>GHMSHWIWQHKDWPHFFWDEKLLSSHLSSARLVQGKLLGIIHTINQQTARQMNAFVLADQAVDTSAIEGEHLNRDSVRSSIANRLGLKQVGINKPVDRYIEGLLDMLLDATENYEQPLTLERLYGWHAALFPTGYSGIHKITVAALRKTDPMQIVSGRPGKIKVHYEAPPSKRVNKEMRIFLNWFNKKDLDGLLRAGIAHLWFELLHPFDDGNGRIGRAIIDLTLAQDEKQNVRYYSLSSAIMQDRKNYYTQLGKSCRGNMDITLWLIWFINCFKTAIHQAFELIDDITLKSRFWEKHATTELNARQIKVLNRLLDAGKKGFIGGMTTRKYTQLTKTSRTTAYRELHDLVLKKCLKPLTKKGRSAAYEIRWVNKEH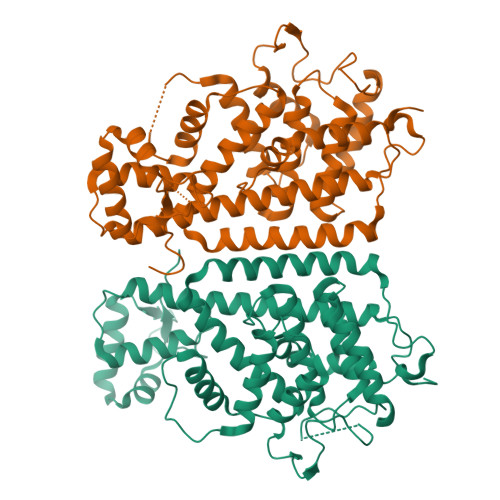KSKK[2x]>MNDLTLSPIAIIHTPYKEKFSVPRQPNLVEDGVGIVELLPPYNSPEAVRGLEQFSHLWLIFQMDQIQQGKWQPTVRPPRLGGNQRVGVFASRATHRPNPLGMSKVELRQVECINGNIFLHLGAVDLVDGTPIFDIKPYIAYADSEPNAQSSFAQEKLPVKMTVEFTEQAKSAVKKREEKRPHLSRFIRQVLEQDPRPAYQQGKPSDRIYGMSLYEFNVKWRIKAGTVNCVEVIEI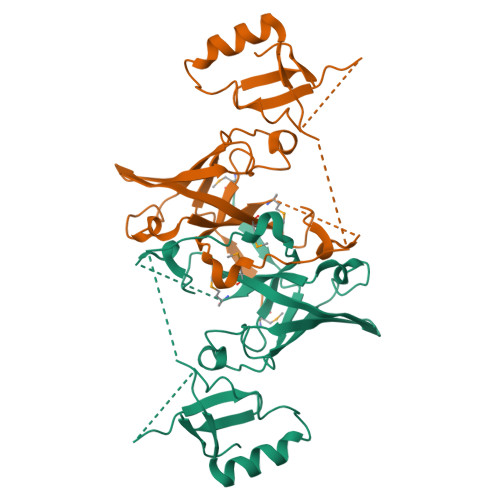EKDKLEHHHHHH[2x]>MGSITENTSWNKEFSAEAVNGVFVLCKSSSKSCATNDLARASKEYLPASTFKIPNAIIGLETGVIKNEHQVFKWDGKPRAMKQWERDLTLRGAIQVSAVPVFQQIAREVGEVRMQKYLKKFSYGNQNISGGIDKFWLEGQLRISAVNQVEFLESLYLNKLSASKENQLIVKEALVTEAAPEYLVHSKTGFSGVGTESNPGVAWWVGWVEKETEVYFFAFNMDIDNESKLPLRKSIPTKIME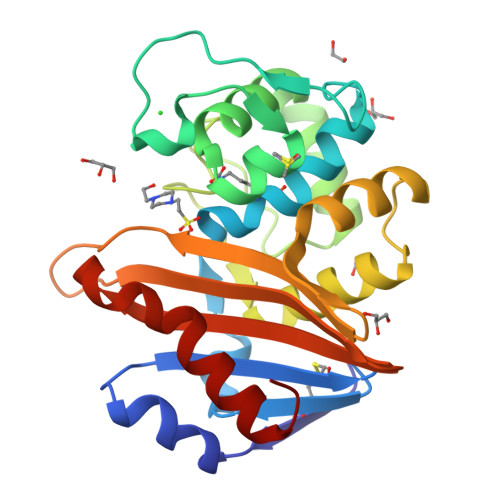SEGII[2x]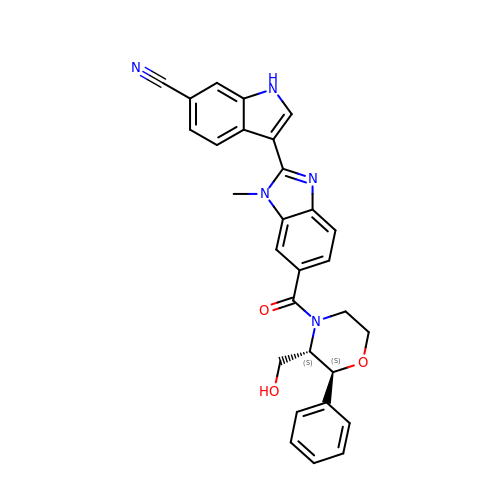3-(6-{[(2S,3S)-3-(hydroxymethyl)-2-phenylmorpholin-4-yl]carbonyl}-1-methyl-1H-benzimidazol-2-yl)-1H-indole-6-carbonitrile | C29 H25 N5 O3 | BFUYKHPXWBXKQQ-SVBPBHIXSA-N> SYKDAYSRINAIVIEGEQEAFDNYNRLAEMLPDQRDELHKLAKMEQRHMKGFMACGKNLSVTPD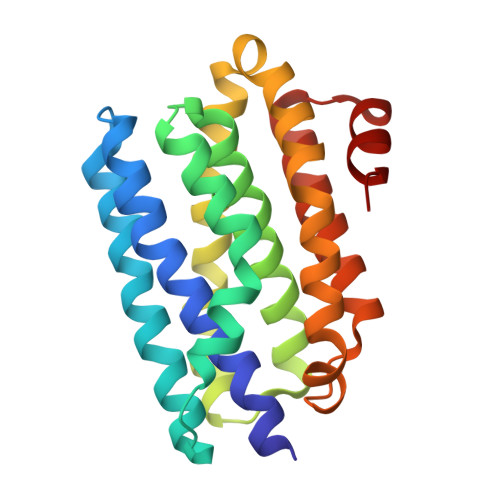MGFAQKFFERLHENFKAAAAEGKVVTCLLIQSLIIECFAIAAFNIYIPVADAFARKITEGVVRDEYLHRNFGEEWLKANFDASKAELEEANRQNLPLVWLMLNEVADDARELGMERESLVEDFMIAYGEALENIGFTTREIMRMSAYG> MRTQGIKPRIREILSKELPEELVKLLPKRWVRIGDVLLLPLRPELEPYKHRIAEVYAEVLGVKTVLRKGHIHGETRKPDYELLYGSDTVTVHVENGIKYKLDVAKIMFSPANVKERVRMA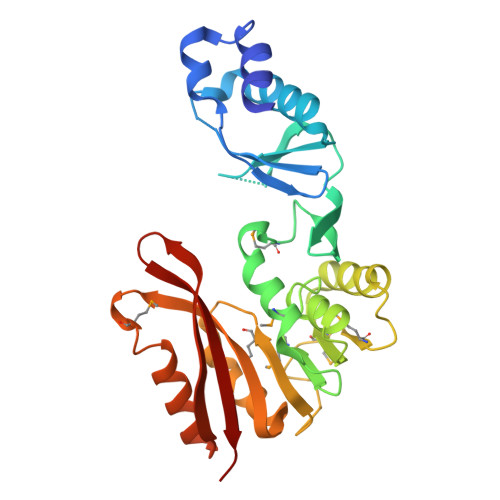KVAKPDELVVDMFAGIGHLSLPIAVYGKAKVIAIEKDPYTFKFLVENIHLNKVEDRMSAYNMDNRDFPGENIADRILMGYVVRTHEFIPKALSIAKDGAIIHYHNTVPEKLMPREPFETFKRITKEYGYDVEKLNELKIKRYAPGVWHVVLDLRVFKS> MNNSEDPFQQVVKDTKEQLNRINNYITRHNTAGDDDQEEEIQDILKD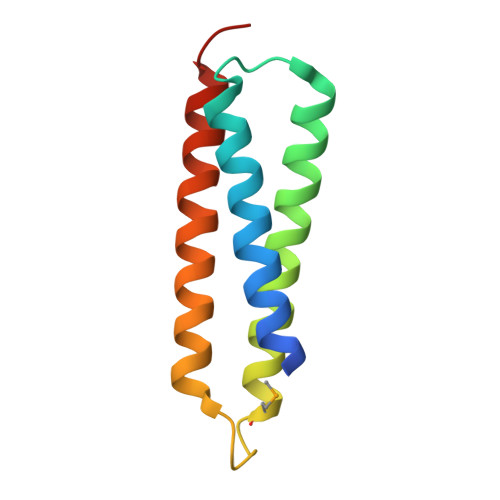VEETIVDLDRSIIVMKRDENEDVSGREAQVKNIKQQLDALKLRFDRRIQESTQT>[8x]SQLTPRRPYLLRAFYEWLLDNQLTPHLVVDVTLPGVQ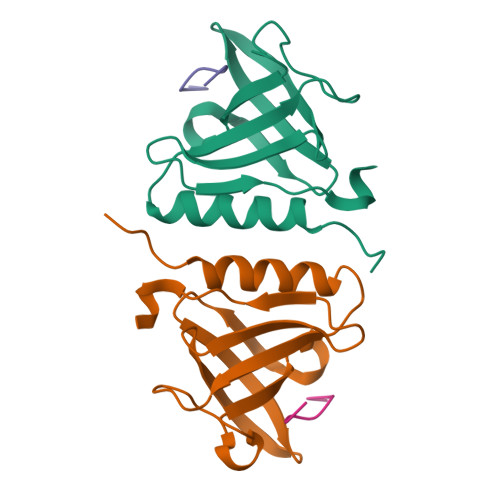VPMEYARDGQIVLNIAPRAVGNLELANDEVRFNARFGGIPRQVSVPLAAVLAIYARENGAGTMFEPEAAYD;>AANDENYA[8x]The key enzyme in the salvage pathway is hypoxanthine–guanine–(xanthine) phosphoribosyltransferase (HG(X)PRT)4. Inhibition of hypoxanthine–guanine–xanthine phosphoribosyltransferase activity decreases the pool of 6-oxo and 6-amino purine nucleoside monophosphates required for DNA and RNA synthesis, resulting in a reduction in cell growth. Five compounds synthesized here that contain a purine base covalently linked by a prolinol group to one or two phosphonate groups have Ki values ranging from 3 nM to >10 μM, depending on the structure of the inhibitor and the biological origin of the enzyme. X-ray crystal structures show that, on binding, these prolinol-containing inhibitors stimulated the movement of active site loops in the enzyme.

The TBrHGPRT1·4 complex refines as a dimer, while the TBrHGPRT1·5 complex refines as two dimers. There is only one difference in the chemical structure of these two ligands, and this is the isomeric attachment of the prolinol ring to the N9 atom of the purine ring. The (R) isomer does once again have the highest affinity (cf. Ki value of 3 nM with 70 nM). As found for 5, the carbonyl oxygen of 4 does not make any interactions in the active site. The difference in their binding, therefore, lies in the positioning of the phosphonate group attached to the nitrogen atom in the prolinol ring. The large electron density found around the phosphonate group attached to the carbon atom in the prolinol ring when 4 binds has been assigned to a magnesium ion. The distances between the metal ion and water and the phosphonyl oxygen agree with the ligation chemistry. Thus, when this compound binds, a magnesium ion is found in an unpredicted locality and assists in binding this ligand.

>[2x]MEPACKYDFATSVLFTEAELHTRMRGVAQRIADDYSNCNLKPLENPLVIVSVLKGSFVFTADMVRILGDFGVPTRVEFLRASSYGHDTKSCGRVDVKADGLCDIRGKHVLVLEDILDTALTLREVVDSLKKSEPASIKTLVAIDKPGGRKIPFTAEYVVADVPNVFVVGYGLDYDQSYREVRDVVILKPSVYETWGKELERRKAAGEAKR>[2x]MGVDPFERNKILGRGINIGNALEAPNEGDWGVVIKDEFFDIIKEAGFSHVRIPIRWSTHAYAFPPYKIMDRFFKRVDEVINGALKRGLAVVINIHHYEELMNDPEEHKERFLALW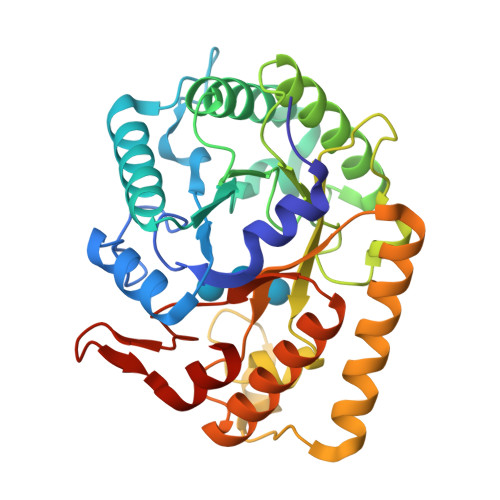KQIADRYKDYPETLFFEILNEPHGNLTPEKWNELLEEALKVIRSIDKKHTIIIGTAEWGGISALEKLSVPKWEKNSIVTIHYYNPFEFTHQGAEWVEGSEKWLGRKWGSPDDQKHLIEEFNFIEEWSKKNKRPIYIGAFGAYRKADLESRIKWTSFVVREMEKRRWSWAYWEFCSGFGVYDTLRKTWNKDLLEALIGGDSIE> VMKTFKEFLLSLDDSVDETEAVKRYNDYKLDFRRQQMQDFFLAHKDEEWFRSKYHPDEVGKRRQEARGALQNRLRVFLSLMETGWFDNLLLDIDKADAIVKMLDAAVIKMEGGTENDLRILEQEEEEEQAGKPGEPSKKEEGRAGAGLGDGERKTNDKDEKKEDGKQAENDSSNDDKTKKSEGDGDKEEKKEDSEKEAKKSSKKRNRKHSGDDSFDEGSVSESESESESGQAEEEKEEAEEALKEKEKPKEEEWEKPKDAAGLECKPRPLHKTCSLFMRNIAPNISRAEIISLCKRYPGFMRVALSEPQPERRFFRRGWVTFDRSVNIKEICWNLQNIRLRECELSPGVNRDLTRRVRNINGITQHKQIVRND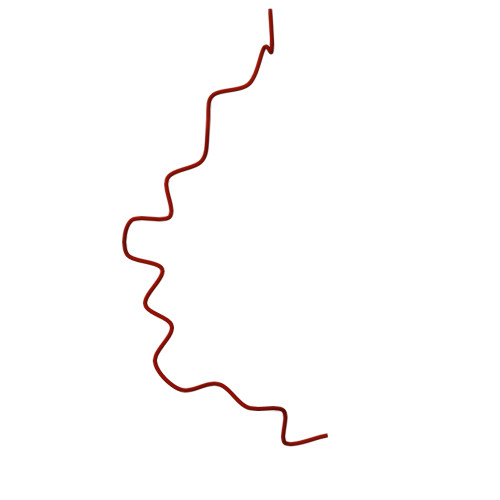IKLAAKLIHTLDDRTQLWASEPGTPPLPTSLPSQNPILKNITDYLIEEVSAEEEELLGSSGGAPPEEPPKEGNPAEINVERDEKLIKVLDKLLLYLRIVHSLDYYNTCEYPNEDEMPNRCGIIHVRGPMPPNRISHGEVLEWQKTFEEKLTPLLSVRESLSEEEAQKMGRKDPEQEVEKFVTSNTQELGKDKWLCPLSGKKFKGPEFVRKHIFNKHAEKIEEVKKEVAFFNNFLTDAKRPALPEIKPAQPPGPAQILPPGLTPGLPYPHQTPQGLMPYGQPRPPILGYGAGAVRPAVPTGGPPYPHAPYGAGRGNYDAFRGQGGYPGKPRNRMVRGDPRAIVEYRDLDAPDDVDFF>MSVSAFNRRWAAVILEALTRHGVRHICIAPGSRSTPLTLAAAENSAFIHHTHFDERGLGHLALGLAKVSKQPVAVIVTSGTAVANLYPALIEAGLTGE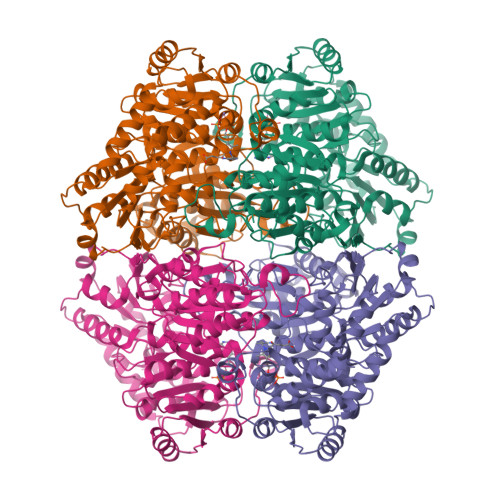KLILLTADRPPELIDCGANQAIRQPGMFASHPTHSISLPRPTQDIPARWLVSTIDHALGTLHAGGVHINCPFAEPLYGEMDDTGLSWQQRLGDWWQDDKPWLREAPRLESEKQRDWFFWRQKRGVVVAGRMSAEEGKKVALWAQTLGWPLIGDVLSQTGQPLPCADLWLGNAKATSELQQAQIVVQLGSSLTGKRLLQWQASCEPEEYWIVDDIEGRLDPAHHRGRRLIANIADWLELHPAEKRQPWCVEIPRLAEQAMQAVIARRDAFGEAQLAHRICDYLPEQGQLFVGNSLVVRLIDALSQLPAGYPVYSNKGASGIDGLLSTAAGVQRASGKPTLAIVGDLSALYDLNALALLRQVSAPLVLIVVNNNGGQIFSLLPTPQSERERFYLMPQNVHFEHAAAMFELKYHRPQNWQELETAFADAWRTPTTTVIEMVVNDTDGAQTLQQLLAQVSHL[8x]> MEKDGLCRADQQYECVAEIGEGAYGKVFKARDLKNGGRFVALKRVRVQTGEEGMPLSTIREVAVLRHLETFEHPNVVRLFDVCTVSRTDRETKLTLVFEHVDQDLTTYLDKVPEPGVPTETIKDMMFQLLRGLDFLHSHRVVHRDLKPQNILVTSSGQIKLADFGLARIYSFQMAL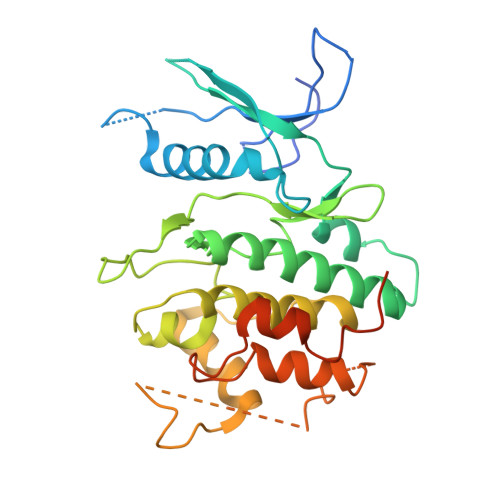TSVVVTLWYRAPEVLLQSSYATPVDLWSVGCIFAEMFRRKPLFRGSSDVDQLGKILDVIGLPGEEDWPRDVALPRQAFHSKSAQPIEKFVTDIDELGKDLLLKCLTFNPAKRISAYSALSHPYFQDLERCKENLDSHLPPSQNTSELNTA> GAMDYSLVKALQTAQQNFVISDPSIPDNPIVYASQGFLTLTGYALSEVLGRNCRFLQGPETDPKAVEKVRKGLERGEDTTVVL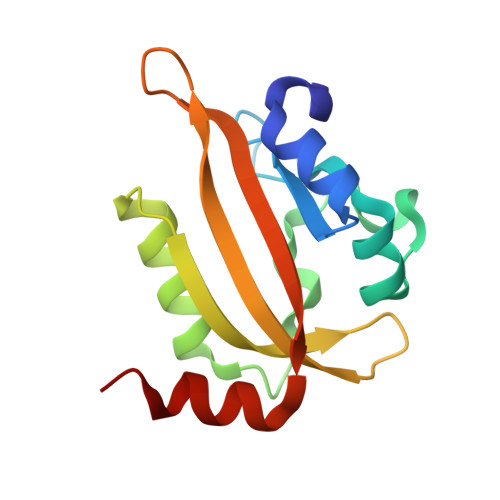LNYRKDGSTFWNQLFIAALRDGEGNVVNYLGVQCKVSEDYAKAFLKNEEN1-O-DEMETHYL-6-DEOXYDOXORUBICIN | C26 H27 N O10 | 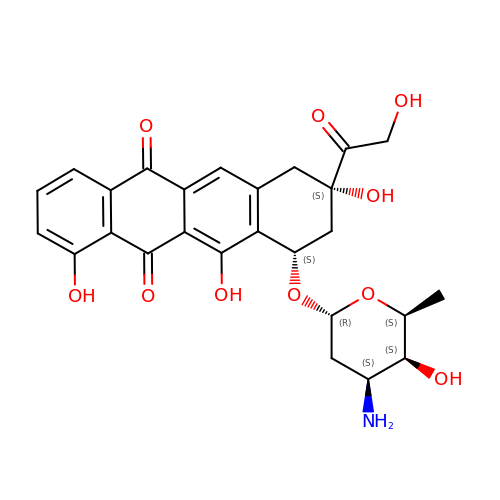ROILTUODAPUWLG-NRFWZUBKSA-N>[2x]MKKILAINFSTASKKGEGTGYAFRKDGQVYVGSIKAYNPKKTAWERTFDIVNAIKDIIDEFDLKGYHLAIETPIMGRNRKHSITLANCNGYFIGAIDGLVNGYTFIDNSKWCSYHLISGKREQRKEESLELLKATGLVDSNCKDDNIADAYNILTYCEHLG

The RuvC from Lactococcus lactis phage bIL67 (67RuvC) was confirmed as a functional Holliday junction resolvase in both in vitro and in vivo experiments. However, unlike EcRuvC, it showed a relaxed structure-specificity, binding and cutting fork and X junctions almost equally well. The 67RuvC enzyme has the classical RNase H fold common to many nucleases and integrases including its cellular EcRuvC counterpart which comprises a central 5-stranded mixed β-sheet (β1–β5) flanked on one side by 2 α-helices (αA and αB) and by 3 on the other (αC, αD and αE). A non-crystallographic dimer is clearly observed in the asymmetric unit of the crystal consistent with symmetrical resolution of Holliday junctions in vitro and the previous cellular RuvC structures.

To investigate the modifications responsible for this difference in structure selectivity, the crystal structure of a 67RuvC D8N mutant was determined at 1.8 Å resolution. This nuclease deficient mutant corresponds to an EcRuvC D7N mutant, which lacks one of four essential catalytic carboxylates, and was chosen to facilitate co-crystallization efforts in the presence of branched and unbranched DNA substrates. Purified 67RuvC D8N was screened for crystallization and well-diffracting crystals obtained in a P-orthorhombic space group subsequently confirmed as P212121. Following unsuccessful efforts to determine the structure of 67RuvC by molecular replacement utilizing models derived from EcRuvC, the structure was solved using phases determined from a selenomethionine-incorporated form of the protein with data collected in a multiwavelength anomalous dispersion (MAD) experiment at three wavelengths. The structural model was refined against a 1.7 Å data set collected at the high energy remote wavelength. The structures presented here, where D8 has been mutated to an asparagine, confirm that these residues are indeed clustered together in a pocket recessed slightly from the surface of the protein, which is partially obscured by a loop formed by residues 12–16. Overall there is no major difference between the structures with and without Mg2+. Residues that come close to the DNA in the junction include R77 and R79, which protrude into the junction centre. The electron density for the side-chains of these residues is weak in the free enzyme structure but it is quite possible that these residues would become ordered when the protein is in complex with the DNA substrate.> MNLPTAQEVQGLMARYIELV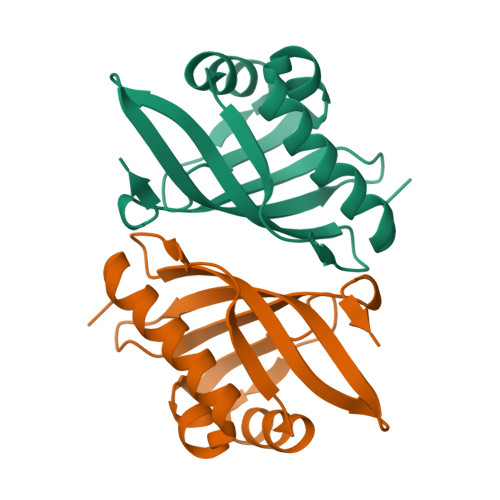DVGDIEAIVQMFADDATVEDPFGQPPIHGREQIAAFYRQGLGGGKVRACLTGPVRASHNGCGAMPFRVEMVWNGQPCALDVIDVMRFDEHGRIQTMQAYWSEVNLSVREPQ> MVLLMGVRRCGKSSICKVVFHNMQPLDTLYLESTSNPSLEHFSTLIDLAVMELPGQLNYFEPSYDSERLFKSVGALVYVIDSQDEYINAITNLAMIIEYAYKVNPSINIEVLIHKVDGLSEDFKVDAQRDIMQRTGEELLELGLDGVQVSFYLTSIFDHSIYEAFSRIVQKLIPELSFLENMLDNLIQHSKIEKAFLFDVNSKIYVSTDSNPVDIQMYEVCSEFIDVTIDLFDLYKAPVLRNSQKSSDKDNVINPRNELQNVSQLANGVIIYLRQMIRGLALVAIIRPNGTDMESCLTVADYNIDIFKKGL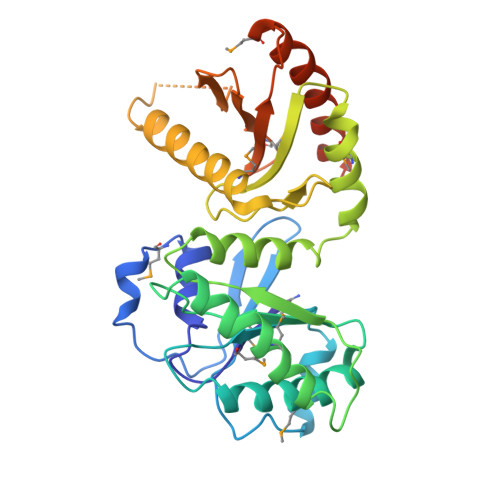EDIWANARASQAKNSIEDDV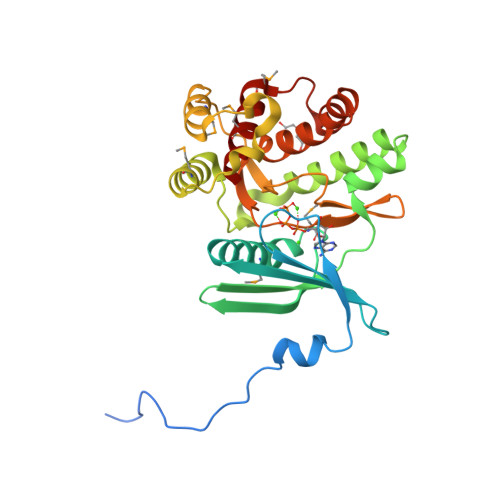>[3x]MGSSHHHHHHSSGRENLYFQGMSHIQRETSCSRPRLNSNLDADLYGYRWARDNVGQSGATIYRLYGKPNAPELFLKHGKGSVANDVTDEMVRLNWLTAFMPLPTIKHFIRTPDDAWLLTTAIPGKTAFQVLEEYPDSGENIVDALAVFLRRLHSIPVCNCPFNSDRVFRLAQAQSRMNNGLVDASDFDDERNGWPVEQVWKEMHKLLPFSPDSVVTHGDFSLDNLIFDEGKLIGCIDVGRVGIADRYQDLAILWNCLGEFSPSLQKRLFQKYGIDNPDMNKLQFHLMLDEFF> PTIQPTQPTTQLPTDSPTQPTTGSFCPGPVTLCSDLESHSTEAVLGDALVDFSLKLYHAFSAMKKVETNMAFSPFSIASLLTQVLLGAGENTKTNLESILSYPKDFTCVHQALKGFTTKGVTSVSQIFHSPDLAIRDTFVNASRTLYSSSPRVLSNNSDANLELINTWVAKNTNNKISRLLDSLPSDTRLVLLNAIYLSAKWKTTFDPKKTRMEPFHFKNSVIKVPMMNSKKYPVAHFIDQTLKAKVGQLQLSHNLSLVILVPQNLKHRLEDMEQALSPSVFKAIMEKLEMSKFQPTLLTLPRIKVTTSQDMLSIMEKLEFFDFSYDLNLCGLTEDPDLQVSAMQHQTVLELTETGVEAAAASAISVARTLLVF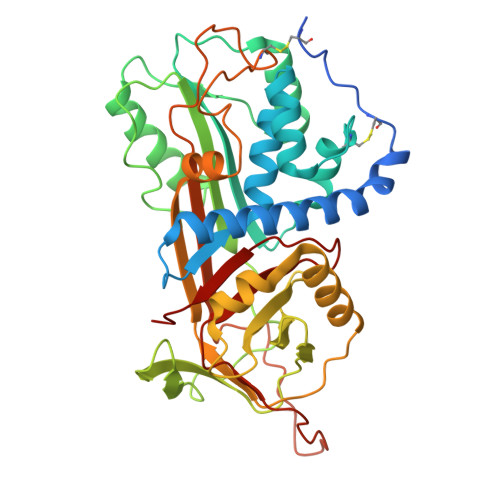EVQQPFLFVLWDQQHKFPVFMGRVYDPRA>[2x]GSHMRGREEKAPEEPQPVKMPENNSVVAATWNAVQLEDSLGMEVGYRLIPMVDFQQDGELLGRIRSIRKKFAQDMGFLPPVVHIRDNMDLQPARYRILMKGVEIGSGDAYPGRWLAINPGTAAGTLPGEKTVDPAFGLDAIWIESALKEQAQIQGFTVVEASTVVATHLNHLIGQFSAELFGRQEAQQLLDRVSQEMPKLTEDLVPGVVTLTTLHKVLQNLLAEKVPIRDMRTILETLAEHAPLQSDPHELTAVVRVALGRAITQQWFPGNEEVQVIGLDTALERLLLQALQGGGGLEPGLADRLLAQTQEALSRQEMLGAPPVLLVNHALRPLLSRFLRRSLPQLVVLSNLELSDNRHIRMTATIGGK

The flagellar protein export apparatus switches substrate specificity from hook-type to filament-type upon hook assembly completion, thereby initiating filament assembly at the hook tip. The C-terminal cytoplasmic domain of FlhA (FlhAC) serves as a docking platform for flagellar chaperones in complex with their cognate filament-type substrates. FlhAC (residues 328–692) consists of four domains, D1, D2, D3, and D4, and a flexible linker (FlhAL) (residues 328–361) connecting FlhAC with the N-terminal transmembrane domain of FlhA. Interactions of the flexible linker of FlhA (FlhAL) with its nearest FlhAC subunit in the FlhAC ring is required for the substrate specificity switching.

We found a new orthorhombic crystal that diffracted up to 2.8 Å resolution, with unit cell dimensions a = 71.7 Å, b = 96.2 Å, c = 114.1 Å and the asymmetric unit containing two FlhAC molecules (A and B). The residues from Val-349 to Val-357 in FlhAL of Mol-A form an α-helix, which interacts with the hydrophobic dimple of a neighboring Mol-A molecule related by a crystallographic symmetry. Trp-354 fits into the hydrophobic dimple, and Ala-351 hydrophobically contacts with Pro-442 on the periphery of the dimple. Ile-7 and Tyr-10 of the N-terminal α-helix of FliS is in the corresponding position of Ala-351 and Trp-354 of FlhAL, respectively. Tyr-10 fits into the hydrophobic dimple of FlhAC, and Ile-7 interacts with Pro-442 of FlhAC. These observations suggest that FlhAL and flagellar chaperones bind competitively to a common binding site on FlhAC and that the dissociation of FlhAL from this binding site is required for the binding of the flagellar chaperones to FlhAC. When Ala-351 and Ala-356 of FlhAC-ED in the crystal structure were replaced back to the original Glu-351 and Asp-356 residues, respectively, the side chain arm of Glu-351 can form a hydrophobic contact with Pro-442, suggesting that FlhAL can bind to the hydrophobic dimple of FlhAC even in the wild type without the flhAED mutation. Because the introduced Ala residues would increase the helical propensity of residues 349–357 of FlhAL as seen in the crystal, we suggest that the flhAED mutation allowed residues 349–357 of FlhAL to efficiently form an α-helix to stabilize the binding of FlhAL to the hydrophobic dimple of FlhAC. Far-UV CD measurements revealed that the flhAED mutation did not affect the secondary structures of FlhAC. These suggest that FlhAC-ED adopts a more compact conformation than wild-type FlhAC. Unlike wild-type FlhAC, FlhAC-ED and FlhAC-EWD did not bind to immobilized GST-FlgN at protein concentrations less than 10 μM, indicating that FlhAL with either of these two mutations inhibits the binding of FlhAC to FlgN.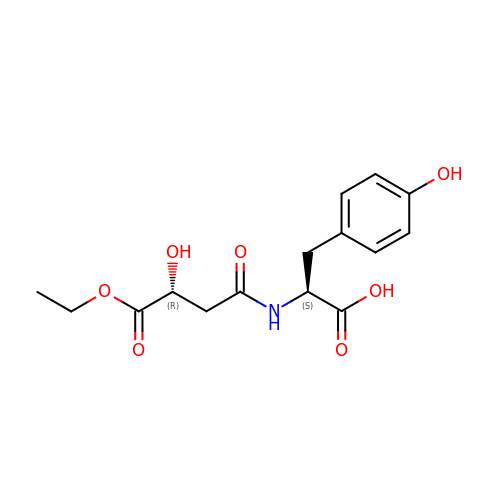N-[(3R)-4-ethoxy-3-hydroxy-4-oxobutanoyl]-L-tyrosine | C15 H19 N O7 | NGFYRWHZMJJCIF-NWDGAFQWSA-N>[2x]GSHMGQSITDYNYKKPLHNDYQILDKSKIFGSNSGSFVMYSMKKDKYYIYNEKESRKRYSPNSTYKIYLAMFGLDRHIINDENSRMSWNHKHYPFDAWNKEQDLNTAMQNSVNWYFERISDQIPKNYTATQLKQLNYGNKNLGSYKSYWMEDSLKISNLEQVIVFKNMMEQNNHFSKKAKNQLSSSLLIKKNEKYELYGKTGTGIVNGKYNNGWFVGYVI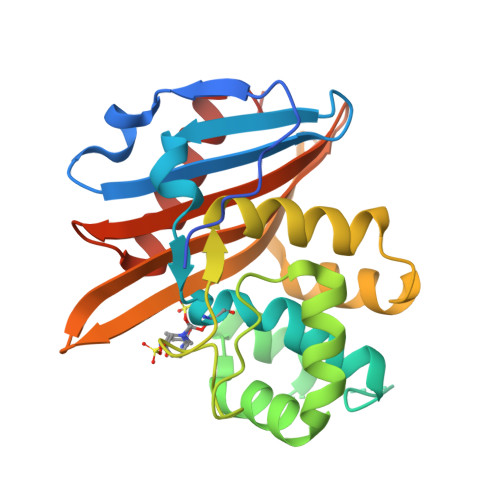TNHDKYYFATHLSDGKPSGKNAELISEKILKEMGVLNGQ>[2x]GPLGSMEPEEYRERGREMVDYICQYLSTVRERRVTPD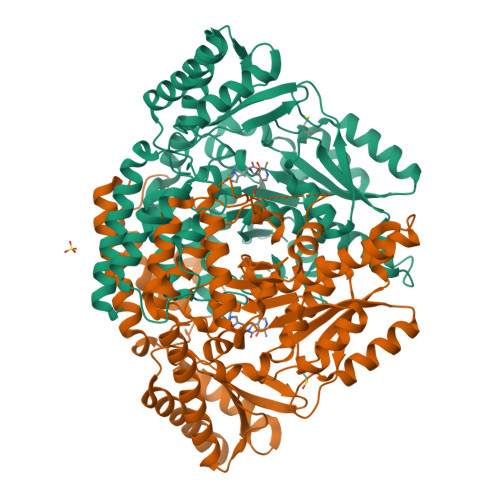VQPGYLRAQLPESAPEDPDSWDSIFGDIERIIMPGVVHWQSPHMHAYYPALTSWPSLLGDMLADAINCLGFTWASSPACTELEMNVMDWLAKMLGLPEHFLHHHPSSQGGGVLQSTVSESTLIALLAARKNKILEMKTSEPDADESSLNARLVAYASDQAHSSVEKAGLISLVKMKFLPVDDNFSLRGEALQKAIEEDKQRGLVPVFVCATLGTTGVCAFDCLSELGPICAREGLWLHIDAAYAGTAFLCPEFRGFLKGIEYADSFTFNPSKWMMVHFDCTGFWVKDKYKLQQTFSVNPIYLRHANSGVATDFMHWQIPLSRRFRSVKLWFVIRSFGVKNLQAHVRHGTEMAKYFESLVRNDPSFEIPAKRHLGLVVFRLKGPNSLTENVLKEIAKAGRLFLIPATIQDKLIIRFTVTSQFTTRDDILRDWNLIRDAATLILSQ>MHHHHHHGARIIYDRAFLMACRGGGGENLYFQGKHPLQNRWALWFFKNDKSKTWQANLRLISKFDTVEDFWALYNHIQLSSNLMPGCDYSLFKDGIEPMWEDEKNKRGGRWLITLNKQQRRSDLDRFWLETLLCLIGESFDDYSDDVCGAVVNVRAKGDKIAIWTTECENREAVTHIGRVYKERLGLPPKIVIGYQSHADTATKSGSTTKNRFVV[2x]

Eukaryotic initiation factor 4E (eIF4E) serves as a regulatory hub for oncogene-driven protein synthesis and is considered a promising anticancer target. The eIF4F complex includes a core of eIF4E, eIF4G and eIF4A5,6. eIF4E recognises and binds the mRNA 5’cap, and recruits eIF4G to provide a scaffold function for the eIF4F complex, while eIF4A is an RNA helicase that is stimulated by binding to eIF4E and eIF4G8. Here we screen a fragment library against eIF4E and identify a ligand-binding site with previously unknown function.

When compound 4 was profiled against the major variant of eIF4E (D127), the protein ligand crystal structure showed a similar binding mode for both variants. A small change in flexible loop conformation (around L85) was observed for the major D127 variant compared to the minor N127 which may in part explain the 5-fold reduction in binding affinity (Kd = 0.09 µM; LE 0.38). Thermodynamically, binding of compound 4 to both eIF4E variants was driven by a large favourable enthalpic contribution with a small entropic penalty. Compound 4 binds tightly to eIF4E, inducing an extension to the α1 helix and a conformational change to the I79 – L85 loop. Comparison of the compound 4-eIF4E structure with that of an eIF4G peptide51 bound to eIF4E suggested that this conformational change would potentially impact on binding of eIF4G due to steric clashes between residues H78-N84 from eIF4E with residues D638-L641 from the eIF4G peptide. Compound 4 treatment disrupted eIF4G binding to eIF4E determined by co-immunoprecipitation with an eIF4E antibody from SW620 human colorectal cancer cell lysates. Consistent with this mode of competitive binding, incubation of cell lysates with a peptide (RIIY; RIIYDRKFLMECRNSPV)56 derived from 4E-BP1 inhibited binding of both eIF4G and 4E-BP1 to eIF4E. This contrasted with compound 4 treatment, which did not disrupt 4E-BP1 binding to eIF4E even when eIF4G binding was lost.>GAMDIVVNDDLSCRFLEGFNTRDALCKKISMNTCDEGDPFFVADLGDIVRKHETWKKCLPRVTPFYAVACNDDWRVLGTLAALGTGFDCASNTEIQRVRGIGVPPEKIIYANPCKQISHIRYARDSGVDVMTFDCVDELEKVAKTHPKAKMVLRISTDDSLARCRLSVKFGAKVEDCRFILEQAKKLNIDVTGVSFHVGSGSTDASTFAQAISDSRFVFDMGTELGFNMHILDIGGGFPGTRDAPLKFEEIAGVINNALEKHFPPDLKLTIVAEPGRYYVASAFTLAVNVIAKKVTPGVQTDVGAHAESNAQSFMYYVNDGVYGS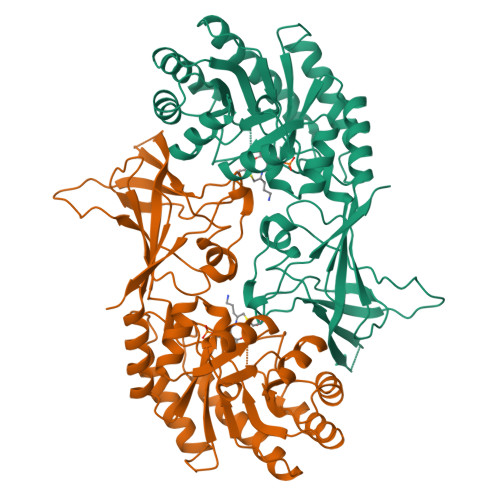FNCILYDHAVVRPLPQREPIPNEKLYPSSVWGPTCDGLDQIVERYYLPEMQVGEWLLFEDMGAYTVVGTSSFNGFQSPTIYYVVSGLPDHVVRELKSQKS[4x]>GVFAFEDEHPSAVAQAKLFKALTKDSDDIIPKVIEQIQSVEIVEGNGGPGTVKKITASHGGHTSYVLHKIDAIDEASFEYNYSIVGGTGLDESLEKITFESKLLSGPDGGSIGKIKVKFHTKGDVLSDAVREEAKARGTGLF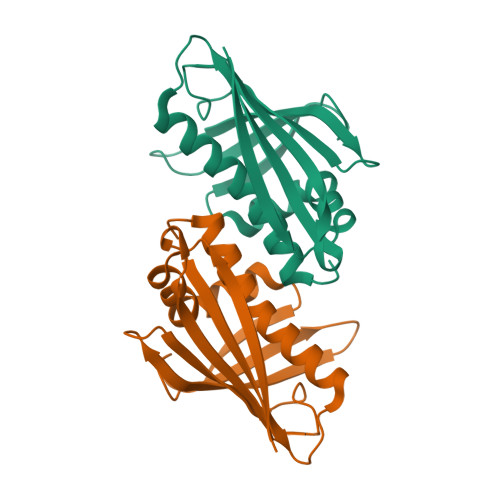KAVEGYVLANPNY[2x]2-[(4~{R})-2',5'-bis(oxidanylidene)spiro[2,3-dihydro-1~{H}-naphthalene-4,4'-imidazolidine]-1'-yl]-~{N}-[4-chloranyl-3-(dimethylsulfamoyl)phenyl]ethanamide 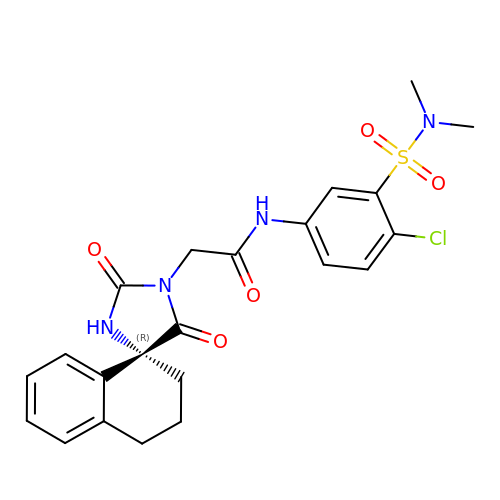| C22 H23 Cl N4 O5 S | MZEQXVHBSVQKGA-JOCHJYFZSA-N> MTRKDPGSSIWFSLAIDGESLGYFNGCEGLSTQVEVEQRQEGGNNGFVWQLPTRVTYSNIRLTRPLTPDTAKVAKWISSVQTGIQRPTAQISALRADGSLVARWGLIDVLPVSWQGPSLDPGSASVANEVLEIAHHGF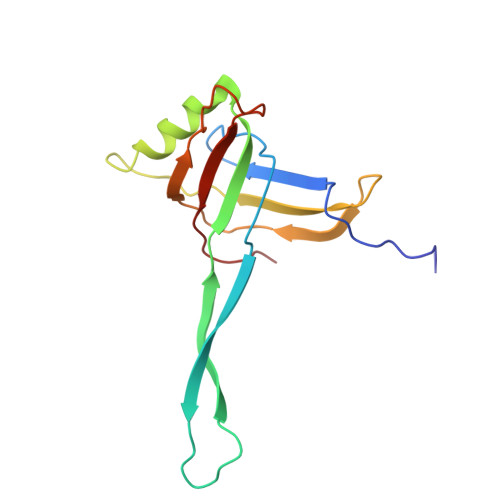TD>AEKPKLHYFNARGRMESTRWLLAAAGVEFEEKFIKSAEDLDKLRNDGYLMFQQVPMVEIDGMKLVQTRAILNYIASKYNLYGKDIKERALIDMYIEGIADLGEMILLLPVCPPEEKDAKLALIKEKIKNRYFPAFEKVLKSHGQDYLVGNKLSRADIHLVELLYYVEELDSSLISSFPLLKALKTRISNLPT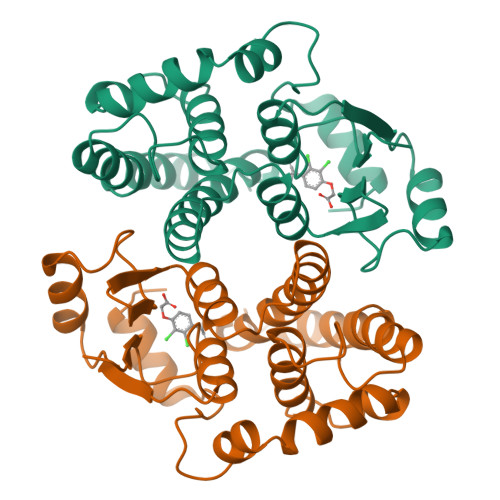VKKFLQPGSPRKPPMDEKSLEEARKIFRF[4x]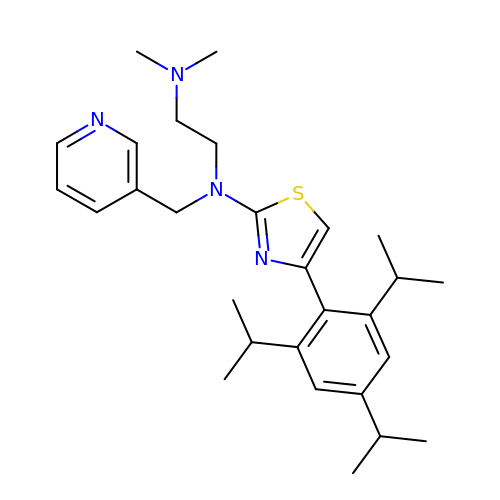N1,N1-dimethyl-N2-[(pyridin-3-yl)methyl]-N2-{4-[2,4,6-tri(propan-2-yl)phenyl]-1,3-thiazol-2-yl}ethane-1,2-diamine | C28 H40 N4 S | VVBFISAUNSXQGZ-UHFFFAOYSA-N>MGSQSTSNHLWLLSDILGQGATANVFRGRHKKTGDLFAIKVFNNISFLRPVDVQMREFEVLKKLNHKNIVKLFAIEEETTTRHKVLIMEFCPCGSLYTVLEEPSNAYGLPESEFLIVLRDVVGGMNHLRENGIVHRNIKPGNIMRVIGEDGQSVYKLTDFGAARELEDDEQFVSLYGTEEYLHPDMYERAVLRKDHQKKYGATVDLWSIGVTFYHAATGSLPFRPFEGPRRNKEVMYKIITGKPSGAISGVQKAENGPIDWSGDMPVSCSLSRGLQVLLTPVLANILEADQEKCWGFDQFFAETSDILHRMVIHVFSLQQMTAHKIYIHSYNTATIFHELVYKQTKIISSNQELIYEGRRLVLEPGRLAQHFPKTTEENPIFVVSRE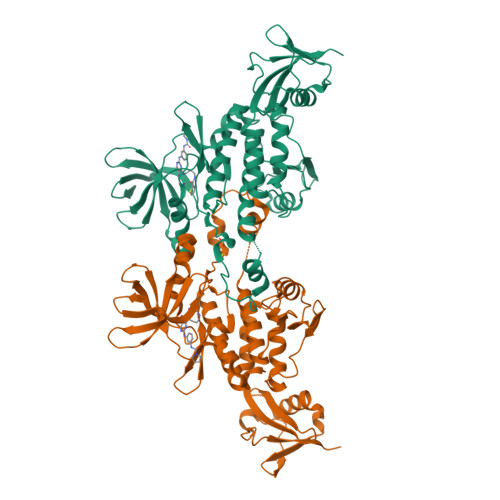GNSHHHHHH[2x]> SIDSALNWDGEMTVTRFDSMTGAHFVIRLDSTQLGPAAGGTRAAQYSNLADALTDAGKLAGAMTLKMAVSNLPMGGGKSVIALPAPRHSIDPSTWARILRIHAENIDKLSGNYWTGPDVNTNSADMDTLNDTTEFVFGRSLERGGAGSSAFTTAVGVFEAMKATVAHRGLGSLDGLTVLVQGLGAVGGSLASLAAEAGAQLLVADTDTERVAHAVALGHTAVALEDVLSTPCDVFAPCAMGGVITTEVARTLDCSVVAGAANNVIADEAASDILHARGILYAPDFVANAGGAIHLVGREVL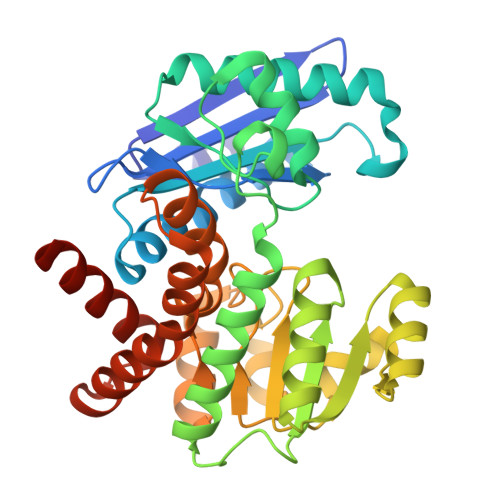GWSESVVHERAVAIGDTLNQVFEISDNDGVTPDEAARTLAGRRAREASTTTATA> PTHIAIALKYNPEKDKAPVVVAKGKGTIAQKIVEIAENYSIPVVRKP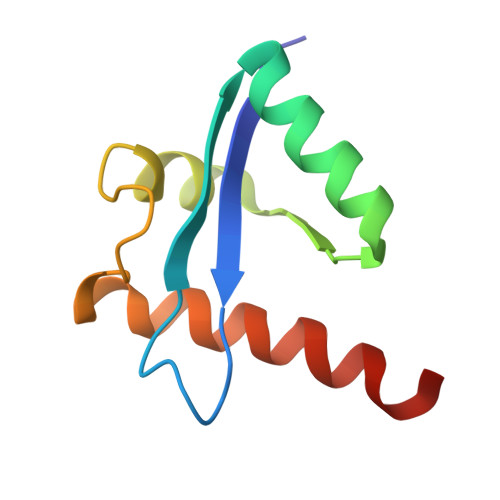ELARALYPAVEVGKEISPKFYKAVAEIIAYVMFKKKKVYA>[3x]MGQIFSRSASPIPRPPRGLAAHHWLNFLQAAYRLEPGPSSYDFHQLKKFLKIALETPARICPINYSL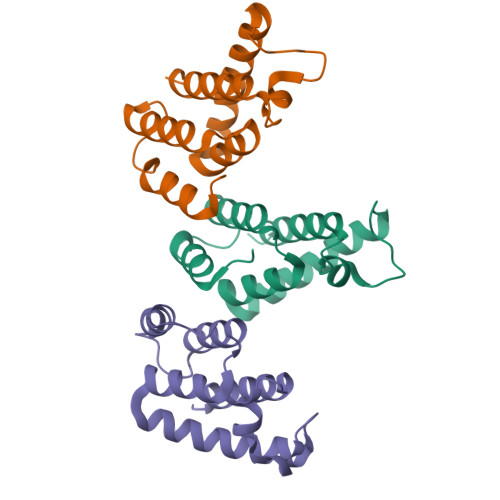LASLLPKGYPGRVNEILHILIQTQAQIPSRPAPPPPSSPTHDPPDSDPQIPPPYVEPTAPQVLPVMHPHGAPPNHRPWQMKDLQAIKQEVSQAAPGSPQFMQTIRLAVQQFDPTAKDLQDLLQYLCSSLVASLHHQQLDSLISEAETRGITGYNPLAGPLRVQANNPQQQGLRREYQQLWLAAFAALPGSAKDPSWASILQGLEEPYHAFVERLNIALDNGLPEGTPKDPILRSLAYSNANKECQKLLQARGHTNSPLGDMLRACQTWTPKDKTKVLVVQPKKPPPNQPCFRCGKAGHWSRDCTQPRPPPGPCPLCQDPTHWKRDCPRLKPTIPEPEPEEDALLLDLPADIPHPKNSIGGEV> MERTELLKPRTLADLIRILHELFAGDEVNVEEVQAVLEAYESNPAE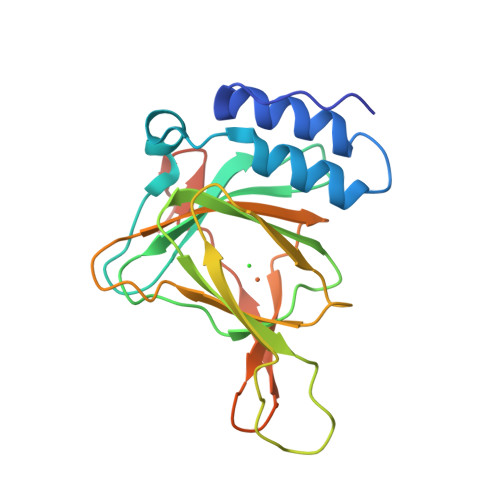WALYAKFDQYRYTRNLVDQGNGKFNLMILCWGEGHGSSIHDHTDSHCFLKLLQGNLKETLFDWPDKKSNEMIKKSERTLRENQCAYINDSIGLHRVENVSHTEPAVSLHLFSPPFDTCHAFDQRTGHKNKVTMTFHSKFGIRTPFTTSGSLENN>[4x]SMRKTIERLLNSELSSNSIAVRTGVSQAVISKLRNGKKELGNLTLNSAEKLFEYQKEMEKVDTWIVYRGRTADMNKSYIAEGSTYEEVYNNFVDKYGYDVLDEDIYEIQLLKKNGENLDDYDVDSDGINNYDKLDEFRESDYVDLEDYDYRELFENSSSQVYYHEFEITHE

AcrIIA15 is an anti-CRISPR (Acr) protein that inhibits Staphylococcus aureus Cas9 (SaCas9). The AcrIIA15 protein, consisting of 170 amino acids, is comprised of two domains: an N-terminal domain (NTD) from residues 1 to 56, which contains a HTH motif resembling a transcriptional repressor, and a C-terminal domain (CTD) from residues 57 to 170. AcrIIA15, by combining the HTH domain and Cas9 inhibitory domain within a single protein, exhibits dual functionality as a bi-functional anti-CRISPR protein capable of both transcriptional repression and CRISPR-based cleavage inhibition. Our structural and biochemical studies demonstrate that AcrIIA15 functions as a dimer to simultaneously inhibit both anti-CRISPR operon transcription and SaCas9-sgRNA DNA recognition.

Based on these findings, we utilized this specific DNA sequence with one base-pair overhangs to form the AcrIIA15-DNA complex for subsequent crystallization experiments. To investigate how AcrIIA15 recognizes promoter DNA in a sequence-specific manner, we determined the crystal structures of the full-length AcrIIA15 or the NTD domain in complex with IR1 DNA at resolutions of 3.15 Å and 3.10 Å, respectively. Resembling a canonical HTH-containing DNA-binding protein, our structural analysis revealed that two AcrIIA15 molecules form a homodimer that binds to a single IR1 dsDNA molecule using its NTD. Each HTH motif of an AcrIIA15 dimer binds to one copy of the IR1 inverted-repeat sequence in a similar manner. The DNA is positioned on the positively-charged surface created by the two HTH domains within the dimer. Importantly, the DNA bound to the AcrIIA15 dimer exhibits a bending angle of approximately 30° compared to typical dsDNA conformations. This observation suggests that the binding of AcrIIA15 induces a conformational change in the DNA, highlighting the specific recognition of the promoter DNA sequence by AcrIIA15. In the AcrIIA15-DNA complex, the HTH motif and the subsequent loop establish extensive interactions with the phosphate backbone of the DNA. Furthermore, EMSA results demonstrated that the R2A mutant exhibited a mild decrease in DNA-binding ability compared to the wildtype, while the L44A and R2A/L44A mutants completely abolished DNA binding. These findings suggest that dimerization is essential for the recognition of dsDNA by AcrIIA15, consistent with the structural observation that the HTH domains of a dimer bind to the inverted-repeat sequence of the DNA.> SMMATITCTRFTEEYQLFEELGKGAFSVVRRCVKVLAGQEYAAKIINTKKLSARDHQKLEREARICRLLKHPNIVRLHDSISEEGHHYLIFDLVTGGELFEDIVAREYYSEADASHCIQQILEAVLHCHQMGVVHRDLKPENLLLASKLKGAAVKLADFGLAIEVEGEQQAWFGFAGTPGYLSPEVLRKDPYGKPVDLWACGVILYILLVGYPPFWDEDQHR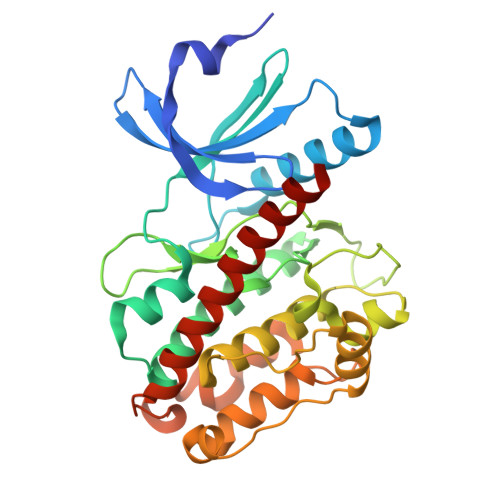LYQQIKAGAYDFPSPEWDTVTPEAKDLINKMLTINPSKRITAAEALKHPWISHRSTVASCMHRQETVDCLKKFNARRKLKGAILAAMLATRNFSG>[2x]MVMDVVSRLHQKYGAEVEKA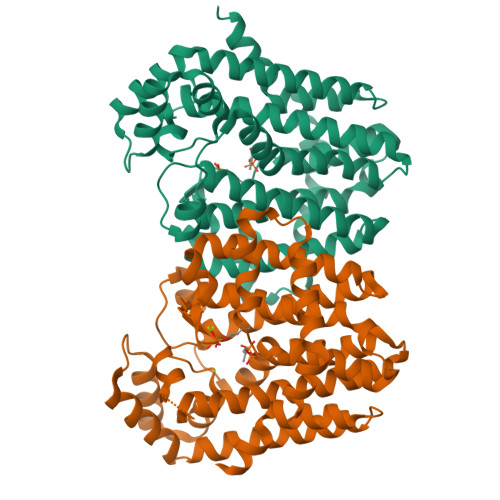LVRYLSIGLAEDFREAVLYQVKTGGKRLRPLLTLAAAEAVSGQWRPALPAAAIVELIHNYSLIYDDIIDRGDVRRGLPTVRKAFGDNAAILVGIWYREAIEEAVLDTPKPTLFAKEVAEVIKAIDEGERLDILFEAAGRSDPYFVQARWREVTLDDYIKMVSLKTGALIAAAAKWGVLSVSDDRGLAEAAWNFGMAAGVAFQIIDDVLDIYGDPKKFGKEIGKDIKEHKRGNAVVAVALSHLGEGERRRLLEILAREVVEEADVREAVALLDSVGAREEALRLAARYREEAERHLAKIPNNGTLKELLDFIVAREYAENLYFQSHHHHHHWSHPQFEK>[4x]MSRVLLVAGGNPSDWPTIEPATYD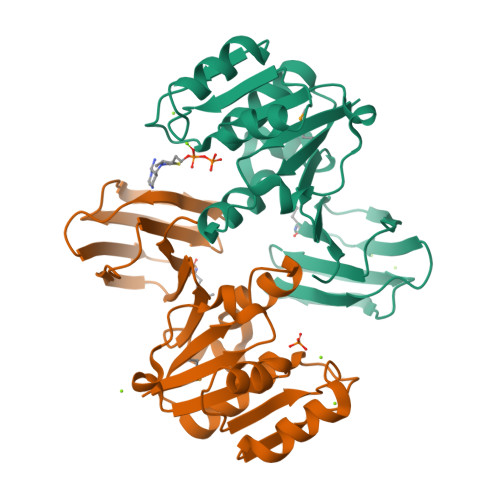YFVGIDRGCLHLLEADLPLQLAVGDFDSLSREEYHFVQETTETLIQAPAEKDDTDTQLALQEALQRFPQAEMTIIGATGGRIDHLLANLWLPFEPRFQGVLRQIRLCDRQNSIQYYAPGSYIVPKEPDKEYLAYCCLTPVENLTLRRSKYLLTNQDVPYPTSYASNEFIEEAAAFSFDAGMIAVIQSKDKLEHHHHHH> MEVEVKLRLLTAAAHLRLTTLLTPYHLKTLHQRNTFFDTPKNDLSLRRAVLRLRFLQNAAVSAASPSPPRCIVSLKAKPTLANGISRVEEDEEEIEYWI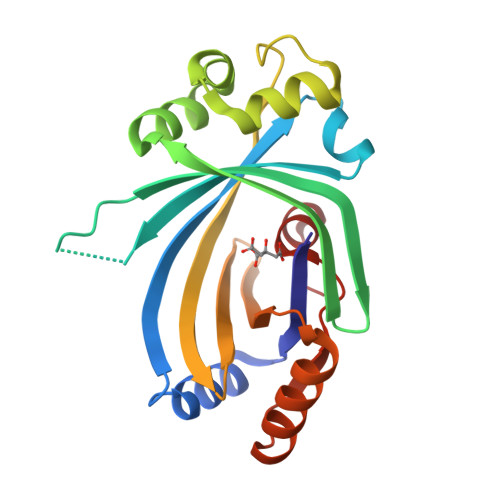GKECVESPAKLSDIGSRVLKRVKEEYGFNDFLGFVCLGGFENVRNVYEWRGVKLEVDETKYDFGNCYEIECETEEPERVKTMIEEFLTEEKIEFSNSDMTKFAVFRSGKLP>[2x]SNAMYKIVSDSACDLSKEYLEKHDVTIVPLSVSFDGETYYRDGVDITRDECYQRMVDDPKLFPKTSLPSVESYADVFRSFVEQGFPVVCFTITTLFSGSYNSAINAKSLVLEDYPDANICVIDSKQNTVTQALLIDQFVRMLEDGLSFEQAMSKLDALMASARIFFTVGSLDYLKMGGRIGKVATAATGKLGVKPVIIMKDGDIGLGGIGRNRNKLKNSVLQVAKKYLDENNKDNFIVSVGYGY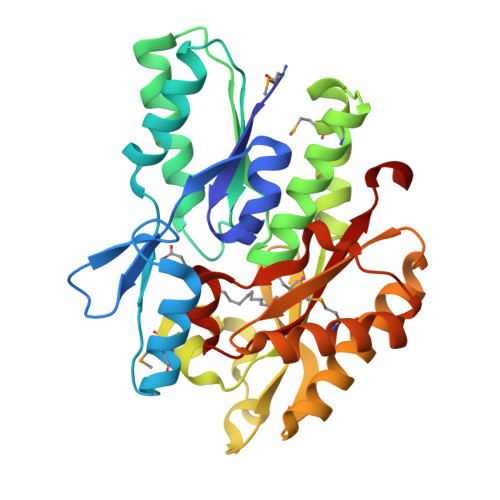DKEEGFEFMKEVESTLDVKLDSETNVAIGIVSAVHTGPYPIGLGVIRKYETL>MSKTQEFRPLTLPPKLSLSDFNEFIQDIIRIVGSENVEVISSKDQIVDGSYMKPTHTHDPTHVMDQDYFLASAIVAPRNVADVQSIVGLANKFSFPLWPISIGRNSGYGGAAPRVSGSVVLDMGKNMNRVLEVNVEGAYCVVEPGVTYHDLHNYLEANNLRDKLWLDVPDLGGGSVLGNAVERGVGYTPYGDHWMMHSGMEVVLANGELLRTGMGALPDPKRPETMGLKPEDQPWSKIAHLFPYGFGPYIDGLFSQSNMGIVTKIGIWLMPNPGGYQSYLITLPKDGDLKQAVDIIRPLRLGMALQNVPTIRHILLDAAVLGDKRSYSSRTEPLSDEELDKIAKQLNLGRWNFYGALYGPEPIRRVLW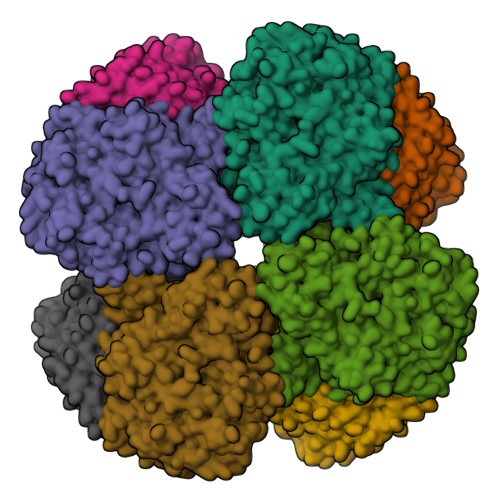ETIKDAFSAIPGVKFYFPEDTPENSVLRVRDKTMQGIPTYDELKWIDWLPNGAHLFFSPIAKVSGEDAMMQYAVTKKRCQEAGLDFIGTFTVGMREMHHIVCIVFNKKDLIQKRKVQWLMRTLIDDCAANGWGEYRTHLAFMDQIMETYNWNNSSFLRFNEVLKNAVDPNGIIAPGKSGVWPSQYSHVTWKL[2x]>[2x]RKPKTGILMLNMGGPETLGDVHDFLLRLFLDRDLMTLPIQNKLAPFIAKRRTPKIQEQYRRIGGGSPIKIWTSKQGEGMVKLLDELSPNTAPHKYYIGFRYVHPLTEEAIEEMERDGLERAIAFTQYPQYSCCTTGSSLNAIYRYYNQVGRKPTMKWSTIDRWPTHHLLIQCFADHILKELDHF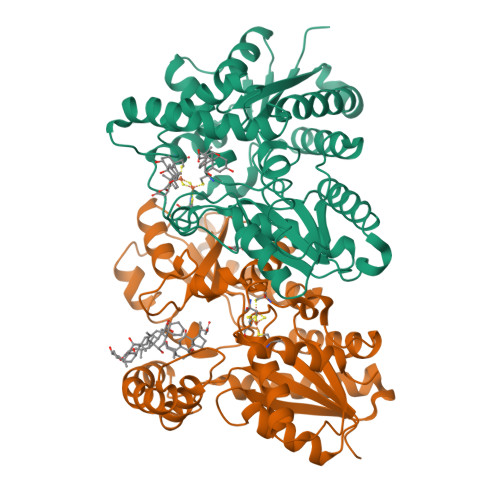PLEKRSEVVILFSAHSLPMSVVNRGDPYPQEVSATVQKVMERLEYCNPYRLVWQSKVGPMPWLGPQTDESIKGLCERGRKNILLVPIAFTSDHIETLYELDIEYSQVLAKECGVENIRRAESLNGNPLFSKALADLVHSHIQSNELCSKQLTLSCPLCVNPVCRETKSFFTSQQL> MGSSHHHHHHSQGSMSLVGSNLHVFTIAELRAVTRDFSMTNFIGEGGFGPVYKGYVHDKTKPGLAAQTVAVRLLDLEGGQGHTEWQTEVFFLGQLRHPHLVKLIGYCYEDEHRLLVYEFMTRGSLEKHLFKKYAASLPWSTRLKIAIGAAKGLAFLHEAEKPVIYRDFKTSNILLDSDYKAKLSDFGLAKDGPEDDETHVSTRVMGTQGYAAPEYIMTGHLTAKSDVYGYGVVLLELLSGRKAVDKTRPPREQSLVEWARPYLTDARRLDRVMDPSLAGQYSTRAAHKAAAVAHQCVALNPKSRPHMSAVVDALEPLLALDDCIVG

We identified ScRIPK, a member of the RLCK VII subfamily, by a screen for sugarcane orthologs of Arabidopsis RIPK and rice GUDK. Thus, ScRIPK is a member of the RLCK VII subfamily localized in the plasma membrane. Furthermore, bacterial growth was measured to determine the bacterial proliferation inside plants, showing that transgenic plants exhibited significantly higher bacterial proliferation than that in wild-type plants at 3 days. These results suggest that ScRIPK plays role in regulating drought tolerance and disease defense in Arabidopsis. Like the typical structure of protein kinases, ScRIPK-KD contains a small N-lobe, composed of five β-sheets and an α-helix, and a large C-lobe, composed of six helices, an activation loop, and a catalytic loop.

In this study, the catalytic base K124–Arginine (K124R) mutation was performed and the mutant protein ScRIPK-KD K124R was purified and crystallized with ATP. The alignment of overall structure between wild type and K124R mutant protein showed no significant conformation changes (root mean square deviation (RMSD) is 1.090 Å comparing 220 corresponding Cα atoms) except for the C-helix and activation loop. The C-helix was outward, away from the active center, and the activation loop had no electron density map. In addition, the position of ATP in protein structure of wild type and K124R mutant, and the crucial residues of ATP binding pocket were partially different. In the ScRIPK-KD K124R mutant structure, Y169 and E170–M172 formed a deep cavity to clamp the adenine group of ATP. Other residues, including G98, G99, and K124, may contribute to the stabilization of the nucleotide through hydrogen bonds. The catalytic spine was also completed by the adenine base of ATP like the wild type. To explore the conformation of this mutant protein, we analyzed whether there was the salt bridge between R124 and E140 and the results showed that there was no salt bridge between them. We also measured the distance of D1 and D2, and dihedral angles of the X-D-F residues, which revealed that the ScRIPK-KD K124R mutant was classified into DFGin group and BLAplus cluster. Furthermore, the regulation spine was analyzed, which was not assembled.> MASMTGGQQMGAPITAYAQQTRGLLGCIITSLTGRDKN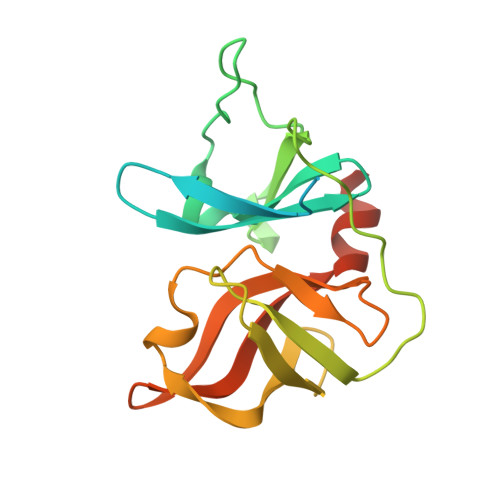QVEGEVQIVSTATQTFLATCINGVCWTVYHGAGTRTIASPKGPVIQMYTNVDQDLVGWPAPQGSRSLTPCTCGSSDLYLVTRHADVIPVRRRGDSRGSLLSPRPISYLKGSSGGPLLCPAGHAVGLFKAAVCTRGVAKAVDFIPVENLETTMRSGSHHHHHH>MILREFCAENLTDLTRLDKAIISRVELCDNLAVGGTTPSYGVIKEANQYLHEKGISVAVMIRPRGGNFVYNDLELRIMEEDILRAVELESDALVLGILTSNNHIDTEAIEQLLPATQGLP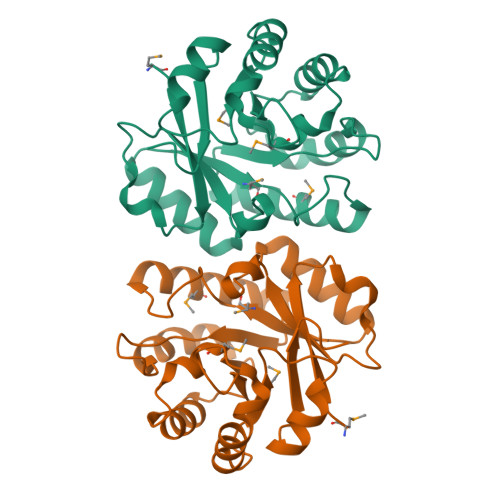LVFHMAFDVIPKSDQKKSIDQLVALGFTRILLHGSSNGEPIIENIKHIKALVEYANNRIEIMVGGGVTAENYQYICQETGVKQAHGTRITQMAGDPLEHHHHHH[2x]At present, the best structurally characterized pLGIC is the G. violaceus ligand-gated ion channel (GLIC), of prokaryotic origin. Each subunit consists of an extracellular domain (ECD), predominantly in a β-sandwich fold, and a transmembrane domain (TMD) composed of four helices, labeled M1–M4. However, the GLIC is a pH-gated channel, activated by lowering the pH, with a maximal activation at pH 4 and a pH50 around 5. We instead found that proton activation is a complex multiple loci mechanism, with the key contribution stemming from the coupling interface between the extracellular and transmembrane domain, with E35 acting as a key proton-sensing residue.

The mutant of the vestibular pair on the β5 strand, D86N-D88N, yields a significant decrease in pH50 greater than 1 pH unit. All residues were also tested individually, with most mutations having no significant effect, although a large majority tend to decrease the pH50 (notably D86N/A, D88N/A, and D91N). Mutation of Asp/Glu residues at the complementary (−) face, in general, decreased the proton sensitivity of the GLIC, with additive effects in many cases, especially for D88 and D86. However, the pattern of phenotypes does not allow discriminating whether those residues are involved in proton sensing or gating, because mutations to Asn/Gln also produced decreased proton sensitivity. A structural analysis was performed on E26Q, E26A, E35Q, E35A, E67A, E75A, E82Q, E82A, D86A, D88N, D88A, H127N, E181A, and H277Q mutants, by solving their structure at pH 4. The key mutants at E26, D86, and D88 were solved at pH 4, each showing a structure similar to that of the Wt. All structures were in the apparently open conformation.

>[5x]GQDMVSPPPPIADEPLTVNTGIYLIECYSLDDKAETFKVNAFLSLSWKDRRLAFDPVRSGVRVKTYEPEAIWIPEIRFVNVENARDAAVVDISVSPDGTVQYLERFSARVLSPLDFRRYPFDSQTLHIYLIVRSVDTRNIVLAVDLEKVGKNDDVFLTGWDIESFTAVVKPANFALEDRLESKLDYQLRISRQYFSYIPNIILPMLFILFISWTAFWSTSYEANVTLVVSTLIAHIAFNILVETNLPKTPYMTYTGAIIFMIYLFYFVAVIEVTVQHYLKVESQPARAASITRASRIAFPVVFLLANIILAFLFFGF> GPDDPLVINGEIEIVTRAPTPAHLADRFDEIRSGWTFRTDDTQALEMDDFENSGMVFVEEARAVWDRPEGTEGKACADCHGAVDDGMYGLRAVYPKYVESAGKVRTVEQMINACRTSRMGAPEWDYIGPDMTAMVALIASVSRGMPVSVAIDGPAQSTWEKGREIYYTRYGQLDLSCASCHEQYFDHYIRADHLSQGQINGFPSYRLKNARLNAVHDRFRGCIRDTRGVPF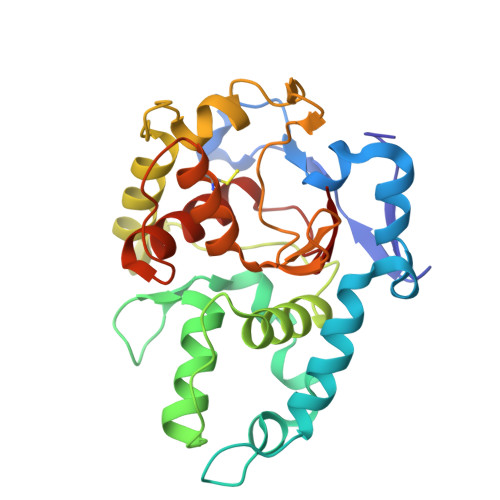AVGSPEFVALELYVASRGNGLSVEGPSVRN>[2x]SMYVIRDEWGNQIWICPGCNKPDDGSPMIGCDDCDDWYHWPCVGIMTAPPEEMQWF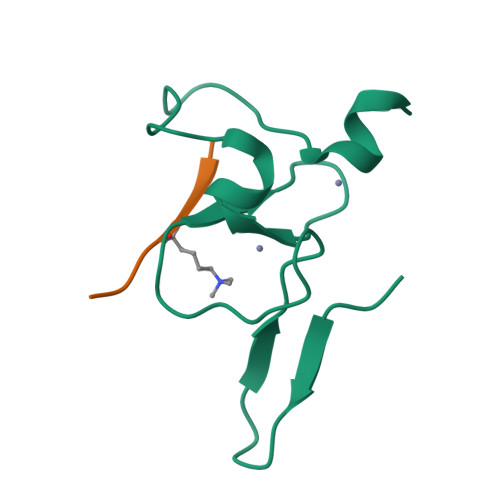CPKCANK;>[2x]ARTKQTA> KPEPTDEEWELIKTVTEAHVATNAQGSHWKQKRKFLPEDIGQAPIVNAPEGGKVDLEAFSHFTKIITPAITRVVDFAKKLPMFCELPCEDQIILLKGCCMEIMSLRAAVRYDPESETLTLNGEMAVTRGQLKNGGLGVVSDAIFDLGMSLSSFNLDD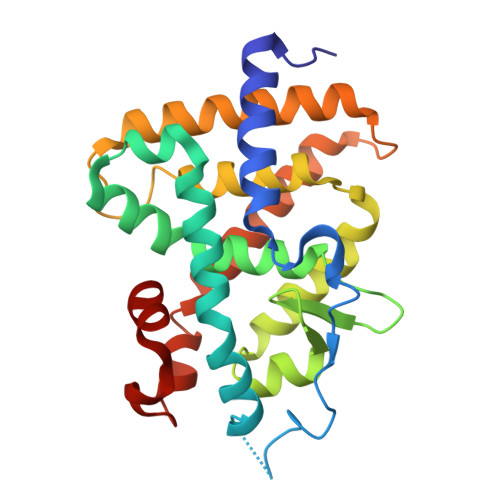TEVALLQAVLLMSSDRPGLACVERIEKYQDSFLLAFEHYINYRKHHVTHFWPKLLMKVTDLRMIGACHASHFLHMKVECPTELFPPLFLEVFE>[2x]GNSIASCADEQPHIGNYR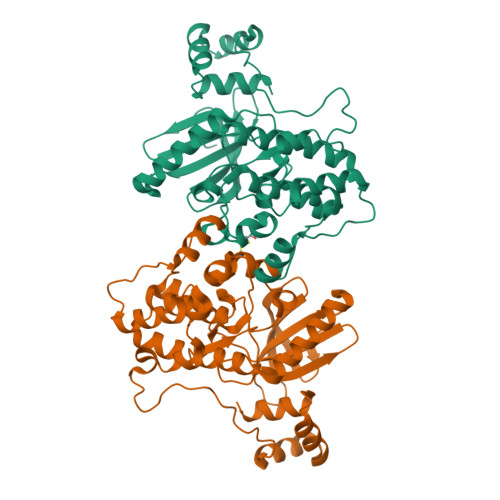LLKTIGKGNFAKVKLARHILTGREVAIKIIDKTQLNPTSLQKLFREVRIMKILNHPNIVKLFEVIETEKTLYLIMEYASGGEVFDYLVAHGRMKEKEARSKFRQIVSAVQYCHQKRIVHRDLKAENLLLDADMNIKIADFGFSNEFTVGGKLDAFCGAPPYAAPELFQGKKYDGPEVDVWSLGVILYTLVSGSLPFDGQNLKELRERVLRGKYRIPFYMSTDCENLLKRFLVLNPIKRGTLEQIMKDRWINAGHEEDELKPFVEPELDISDQKRIDIMVGMGYSQEEIQESLSKMKYDEITATYLLLGRK>MWSHPQFEKAPTATQEPVPVPVTSKAAPSHGYVHPTDILPSGWPTATDLSGGAQPRRFEGTIFDVMTRGTIPKELHGTFYRIMPDYAQPPTYYKGGELNAPIDGDGTVAAFRFKDGKVDYRQRFVETDRFKVERRARKSMYGLYRNPYTHHPCVRQTVESTANTNVVMHAGRFLAMKENGNAYEMDPHTLKTLGYNPFNLPSKTMTAHPKQCSVTGNLVGFGYEAKGLATKDVYYFEVDPSGKVVRDLWLEAPWCAFIHDCALTPNYLVLMLWPFEANLERMKAGGHHWAYDYTKPITWITIPRGAKSKDEVKYWHWKNGMPIHTASGFEDEQGRIIIDSSLVHGNAFPFFPPDSDEQKKKQEADGTPKAQFVRWTIDPRKDNNEQLPDPEVILDTPSEFPQIDNRFMGVEYSSAFINVFVPDRSDGNKNVFQGLNGLAHYKRKEGTTEWYYAGDNCLIQEPVFSPRSKDAPEGDGFVLAIVDRLDLNRSEVVVIDTRDFTKAVAAVQLPFAIRSGIHGQWIPGEVTPDFETKGLVDLPKEEHWAPLSQSPYDPDA[2x]

Herein, Moesziomyces aphidis DSM 70725 aromatic dioxygenase (MapADO) is characterized through X-ray crystallography, biophysical as well as biochemical assays, substrate docking and mutagenesis. MapADO features a seven-bladed β-propeller fold and a Fe2+ center coordinated by four histidine residues and shares a conserved structural motif with homologous enzymes despite low sequence identity (<38%). Similar proteins were termed aromatic dioxygenase (ADO), , apocarotenoid or alkene cleaving oxygenase (ACO). These enzymes primarily act on aromatic compounds with a hydroxy group in 4-position and use a mononuclear Fe2+ iron that is embraced by four histidines. O2 is activated by this nonheme iron and reacts with the C–C double bond of a substrate, eventually leading to C–C bond scission and two carbonyl species as the reaction products.

By analyzing the protein structure both in its native form and in complexes with vanillin 1, 4-hydroxybenzaldehyde (HBA, 3), and ortho-vanillin 5, we uncover the nuances of ligand binding and coordination within MapADO’s active site. MapADO was cocrystallized with excess (40-fold mol) ligands 3 and 1 (products of 3a and 1a cleavage, respectively). The ligands are well-described by their respective electron densities. K169 also stabilizes 1 by interacting with its methoxy oxygen. Adding equimolar 1 reduced 1a conversion by 60%, whereas 5a and 5 showed minor inhibitory effects (12% and 25%, respectively), pointing at higher affinity for 1 over its ortho-isomer. MapADO’s interaction with ligands 4-hydroxybenzaldehyde, ortho-vanillin and vanillin indicate that hydrogen-bonding of the phenolic OH group is key to activity. Structural analysis and site-directed mutagenesis indicate that two key residues (Y136 and K169), and the substrate’s hydroxy group, are essential for accurately positioning the double bond toward the activated oxygen at the Fe center. Fe2+ is coordinated to H200, H251, H316, and H510 and a water molecule. The sixth coordination site is occluded by T156.>MAHAGRTGYDNREIVMKYIHYKLSQRGYEWDAGDDVEENRTEAPEGTESEVVHLTLRQAVDDFSRRYRRDFAEMSSQLHLTPFTARGRFATVVEELFRDGVNWGRIVAFFEFGGVMCVESVNREMSPLVDNIALWMTEYLNRHLHTWIQDNGGWDAFVELYGPSMR[2x]

BCL-2 is the founding member of the pro-survival class of proteins that includes BCL-XL, BCL-W, A1/BFL-1 and MCL-1. They exert their pro-survival function by binding and restraining related members of a family of pro-apoptotic proteins—the sensors of cellular stress (the BH3-only proteins) and the effectors of apoptosis (BAX and BAK). Four or more hydrophobic amino acids on successive helical turns within the BH3 motif engage complementary pockets (P1 through P4) in this surface groove of pro-survival proteins. Venetoclax competes with pro-apoptotic BH3 motifs for BCL-2 binding, releasing pro-apoptotic proteins and allowing apoptosis in cells primed for death.

S55746 is another BCL-2 selective antagonist that has progressed to the clinic. We show here that S55746 also loses potency (~100-fold) against the BCL-2 G101V mutant and we sought a structural explanation for this. To further investigate this we solved the structure of BCL-2 G101V bound to S55746. We obtained diffraction to 2.0 Å in a P 21 spacegroup with two molecules in the asymmetric unit. The orientation of S55746 in the BCL-2 G101V:S55746 complex structure is conserved relative to the WT structure. S55746 inserts a 4-hydroxyphenyl moiety into the P2 pocket but does not insert as deep into the pocket as the corresponding chlorophenyl from venetoclax. This shallow insertion allows the BCL-2 F112 on the α3 helix to insert into the BCL-2 groove extending the P3 pocket. In both BCL-2 WT and BCL-2 G101V structures compared with S55746 E152 is shielded from the base of the P2 pocket by the insertion of F112 into the groove. However, in the BCL-2 G101V:S55746 structure E152 is in an unconventional rotamer, which shows most similarity to tp10, with the Cγ deviating by 40º from the conventional tp10 rotamer. Consistent with this the combination of the G101V mutation with the E152A mutation did not fully restore WT binding to S55746, in contrast to venetoclax, suggesting additional structural features underlying affinity in this case.> MGEKLELRLKSPVGAEPAVYPWPLPVYDKHHDAAHEIIETIRWVCEEIPDLKLAMENYVLIDYDTKSFESMQRLCDKYNRAIDSIHQLWKGTTQPMKLNTRPSTGLLRHILQQVYNHSVTDPEKLNNYEPFSPEVYGETSFDLVAQMIDEIKMTDDDLFVDLGSGVGQVVLQVAAATNCKHHYGVEKADIPAKYAETMDREFRKWMKWYGKKHAEYTLERGDFLSEEWRERIANTS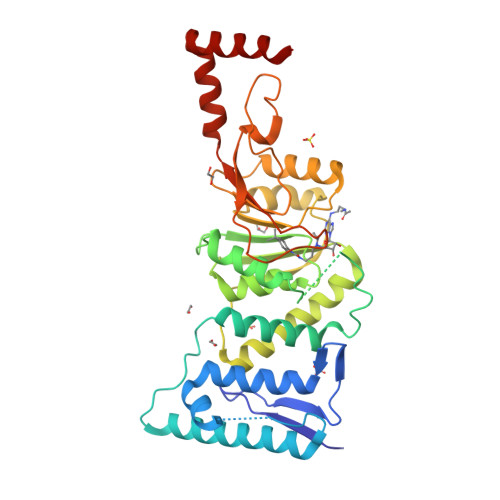VIFVNNFAFGPEVDHQLKERFANMKEGGRIVSSKPFAPLNFRINSRNLSDIGTIMRVVELSPLKGSVSWTGKPVSYYLHTIDRTILENYFSSLKNPKLREEQEAARRRQQR> NLE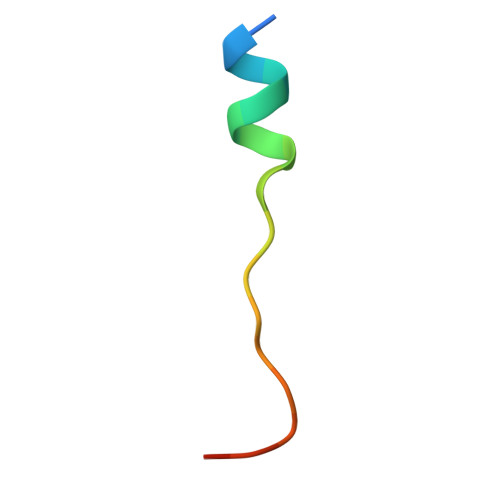VAEYLLQHGADVNAQDK> MGDTKEQRILRYVQQHAKPGDPQSVLEAIDTYCTQKEWAMNVGDAKGQIMDEVIQEHNPSLVLELGAYCGYSAVRMARLLSPGARLLTMEKNPDYAAITQQMLNFAGLQDKVTILIGASQDLIPQLKKYDVDTLDMVFLDHWKDRY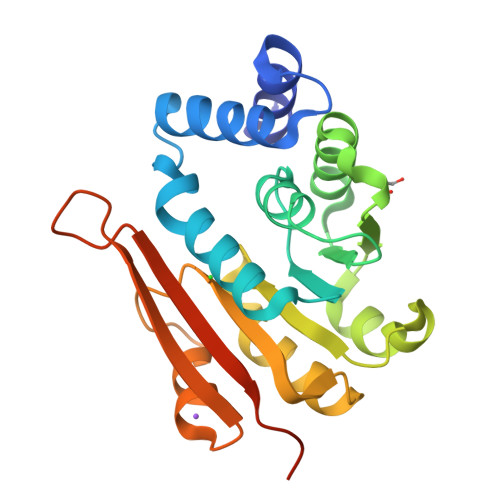LPDTILLEECGLLRKGTVLLADNVIVPGTPDFLAYVRGSSSFECTHYSSYLEYMKVVDGLEKAVYKGPSSPKQPLEHHHHHH>MGTDMSAQAIIRELGLEPHPEGGFYHQTFRDKAGGERGHSTAIYYLLEKGVRSHWHRVTDAVEVWHYYAGAPIALHLSQDGR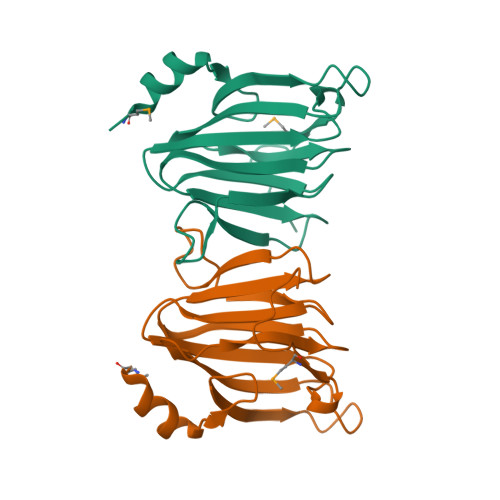EVQTFTLGPAILEGERPQVIVPANCWQSAESLGDFTLVGCTVSPGFAFSSFVMAEPGWSPGDAPLEHHHHHH[7x]Myxopyronin B | C24 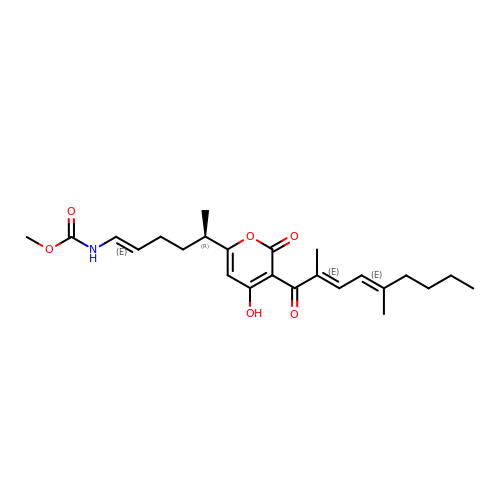H33 N O6 | SPQDIDVJAZFBRL-WXFBSNOUSA-N>[4x]WEEEDVICDGCNGPVVGTRYKCSVCPDYDLCSVCEGKGLHRGHTKLAFPSPFGHLSEGFS

Intriguingly, the autophagy adapter p62/SQSTM1/Sequestosome-1 was recently reported to recognize N-degrons, the N-end rule substrates of the well-characterized UPS, and where ultimately these substrates are delivered to ALS8,9. p62 is a key selective autophagy adapter that plays a role in the degradation of various cellular constituents such as misfolded proteins and their aggregates, malfunctioning organelles, and invading pathogens. Intriguingly, it was recently reported that the central ZZ-domain in p62 plays a critical role in the recognition of N-terminal arginylated BiP/GRP78 by the Arg-tRNA transferase ATE1. Here, we present the high resolution structures of the ZZ-domain of p62 in complex with 8 different N-degrons including type-1 and type-2, and subsequently identify key determinants involved in the unusual recognition.

However, a recent report has shown that the ZZ-domain of p62 also recognizes type-2 N-degrons, although with weaker affinity than with type-1 N-degrons. Therefore, we determined the structure of the ZZ-domain in complex with a variety of N-degrons comprising three type-1 N-degrons and five type-2 N-degrons. As described for the R-BiP complex, two aspartic acid residues, Asp129 and Asp149, bind to the α-amino group, and Asp147 forms a hydrogen bond with the first peptide bond, which means that these interactions are conserved in all different N-terminal residues. However, the side chain of the N-terminal residue of the N-degron is recognized differently. The side chain of Asn132 which undergoes a conformational change plays a critical role in interacting with the first residue of the N-degron. The bipolar nature of the side chain atoms (O and N) of Asn132 allow for the recognition of positively charged type-1 substrates as well as type-2 substrates, and especially N-terminal tyrosine and tryptophan residues since they possess polar atoms in the side chain. As expected, arginine at the primary position showed the strongest binding affinity with, intriguingly, tyrosine and tryptophan residues following in second and third place, respectively. Our structural and biochemical measurement data showed that the presence of tyrosine or tryptophan at the primary position resulted in relatively high affinity because these side chains contain polar atoms, oxygen in tyrosine and nitrogen in tryptophan that can form hydrogen bonds with the side chain of Asn132 of the ZZ-domain. Our structural information clearly explains the affinity measurement data as well as previous pull-down assay results showing that type-1 N-degrons and only a subset of type-2 N-degron peptides (Phe, Trp, and Tyr) displayed binding affinity with p62.>SNAMSDGTILTIKRPITVRAVVTPTWKEEAEREISNGIANADQQLAQLEQEGQTVVDQVRRQSANPLDPRVQEQVANIQQQVAGKRSELEEQKRNLLQQQAQVRELEMDQIVEQGQLESSCEIKVGDNL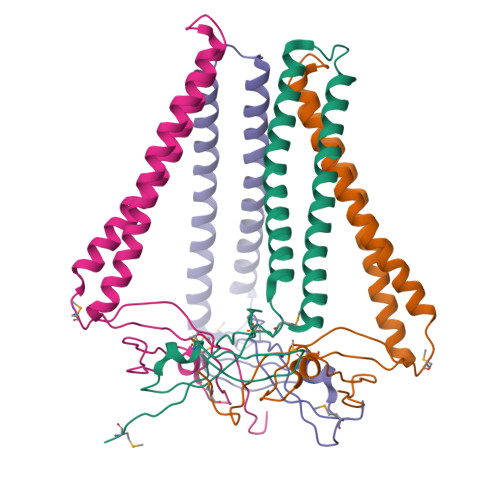VEKMQVAIVVRDGVIQSIEEA[8x]>[2x]SKPKQPPDASPANLLTSLVRAHLDSGPSTAKLDYSKFQELVLPHFGKEDAGDVQQFYDLLSGSLEVIRKWAEKIPGFAELSPADQDLLLESAFLELFILRLAYRSKPGEGK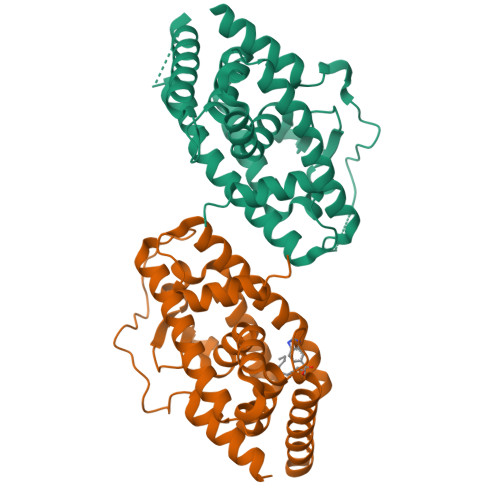LIFCSGLVLHRLQCARGFGDWIDSILAFSRSLHSLLVDVPAFACLSALVLITDRHGLQEPRRVEELQNRIASCLKEHVAAVAGEPQPASCLSRLLGKLPELRTLCTQGLQRIFYLKLEDLVPPPPIIDKIFMDTLPF>MKPSTINQTSRHESMDAILQDVKTTILQTNEIERFAVFSREKTIRPRPYHLSHLFLDKHIEQEAAAEAIQTQKAVPALADMPPALSYGGDLDVTQGAQTLQDVLTEAAKTTNGLTYIVNSKNELTQSYAQLQGDAERVLTGLRALGLKAGDPVFFQFSSNHAMVTAFWACVLGGFVPTLVSAAPTYREMNAAVKKLHHAWKLLEHPLILTDDSLIEEVQGLAFLWHTDQLRVAAVEPMLTLERDTAAHPAAPDDSVFFILTSGSTGMPKCVEHSHRSVLANVKGTVAANQFT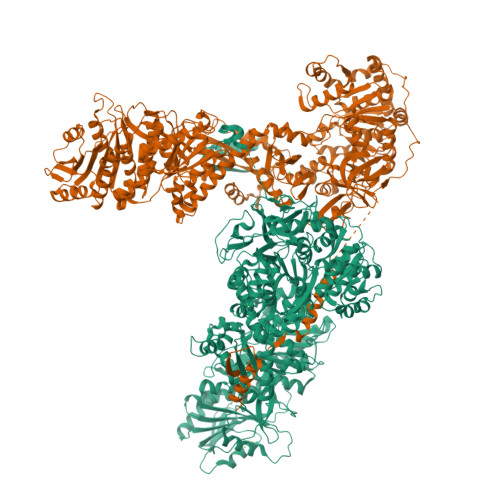QEDVSLDWMPLDHIGGIVMFHLVNVYTGCEQIRARTDDFIAQPLRWLDWMDRYRATKTWAPNFAFAMINDYEKEISSGSWDLSAMTCMINGAEAVVPKTIHRFLHLLAPHGLKGDVIRPAFGMSEISSAVVFSFAIERGDENSGVLTFEETSLTEQLRPAEARETGTVSFTELGKPIPGITIRIVNHQHELLPEDHIGRVQIKGPTTMKGYYRNDEANQEVFQADGWFHTGDLGFLHEGRLTLTGREKDMIIINGKNYHNYEIEAIAEEVPGVETSFVAACSVRMEASASDELILFFTPKLYEPAYIMRASQHIKSHIATKMGLSASRIIPVQKHAFPKTSSGKIERAQLKTRWQEGEFDEMIMEMDMRLENEHTLPNWSYQKKWIPAPLDAADKQIVGDVVIFADPLGLADQLKSFANSEQTYITVEPGQAFKQLTHTHFIIHPNRPSDYEQLFETLRSYGVSVKHIIHLWNYTNQEDKLYVSKAKQAQKTGSMSALFLTKAISVYEEQVAITFVSTHAMNVPEDHIHDVEKATTAGLMTAVQHEWPFIKVQCLDFSLAESVSSHSHAMAMMAELTHDQDCHVAAYRQGVRYIPFLAPLHLEKEQKRKEPPFESSGLYVITGGLGGIGRLVSEQLLTSYQAHLVLLGRKEREALSSDQQETLSLLEKQAKVHGGKVLYEKADITAEKEVEAIISRHEVAGNRRLDGIIHFAGIIQEELLADMTSVSLNDMYEAKVYGTIALHEAASKRRNVLFLSSSSARTLKGGMTVGAYCAANEFVEQFAHYQKLTSTVKPYCFSFSMWDEIGMSEGSMIKGMLKERGYLPISKQAGFQTMLACLMTDAPLIYTGLDRSKKEIHEMIHADAEMQTEQTFYVFFKTDQTKAVEERLYQSIHTCLQSRLSGEYAVHLFPEEYWKETEDGSPDEAYFHELIEESGMDADNRAPHTETEKLLAHIWSELLDVSDVSCGDHFFLLGGHSLKATQMLSAVRQKTGFDVPLAVLFEHTRLGELADWIDSNAKADEVIPMRAAAENLYFQ[4x]>[9x]MIELEFHDVAANTSSTFDPEVAYANFKRVHTTGLSYDHIRIFYIKGREIKTSLAKRSEWEVTLNLGGWKITVYNTNFPGNRNNPVPDDGLTLHRLSG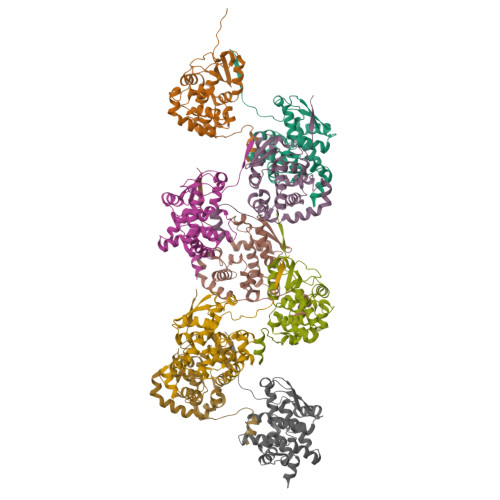FLARYLLEKMLKVSEPEKLIIKSKIINPLAEKNGITWNDGEEVYLSFFPGSEMFLGTFRFYPLAIGIYKVQRKEMEPKYLEKTMRQRYMGLEAATWTVSKLTEVQSALTVVSSLGWKKTNVSAAARDFLAKFGINM> SAIKPDMKIKLRMEGNVNGHHFVIDGDGTGKPFEGKQSMDLEVKEGGPLPFAFDILTTAFLYGNRVFAKYPDNIQD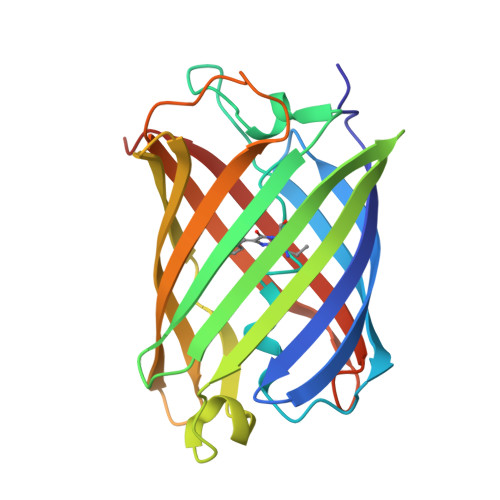YFKQSFPKGYSWERSLTFEDGGICNARNDITMEGDTFYNKVRFYGTNFPANGPVMQKKTLKWEPSTEKMYVRDGVLTGDVEMALLLEGNAHYRCDFRTTYKAKEKGVKLPGAHFVDHCIEILSHDKDYNKVKLYEHAVAHSGLPDNARR>MGSERTCCPVNWVEHERSCYWFSRSGKAWADADNYCRLEDAHLVVVTSWEEQKFVQHHIGPV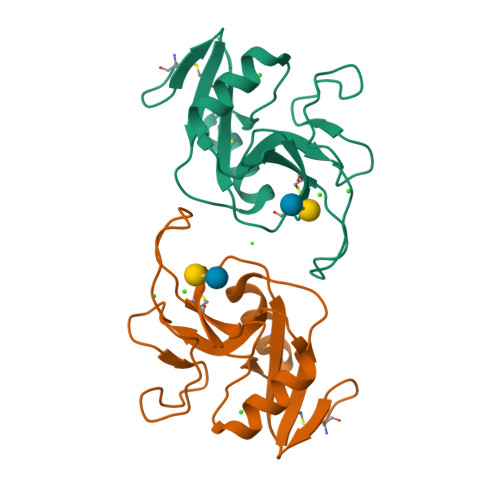NTWMGLHDQNGPWKWVDGTDYETGFKNWRPEQPDDWYGHGLGGGEDCAHFTDDGRWNDDVCQRPYRWVCETELDKASQEPPLL[2x]>[2x]MSKQGLTAGLAEAVRTSQPEHSVDAIRKAKKGLLDFTAASFAGR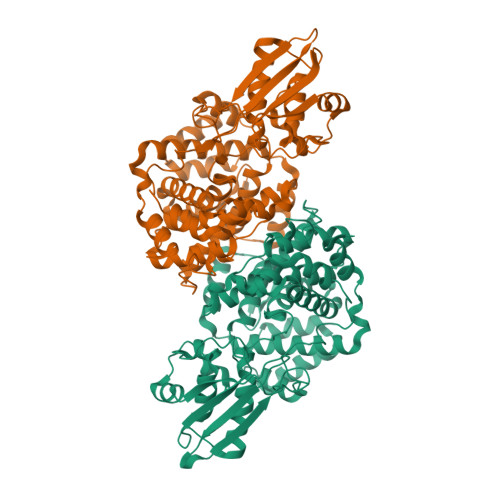EDKGIQKLLRLIEDEGGRPLVPIIGQGKKAAPLQSAMLNGFIAHALDFDDVHSDVRGAPSAVIVPALIASAARGHDERLLGAYIVGVEVMARLGESIGSRHYEKGWHNTGTLGAIAAACAVGYAEELTQEELEKAIGFAATQSAGMRVQFGTEMKPLHAGLAAQAGLLAVKLAQSEFGGSRTAFDGETGFFSLYGDVEKAQHTLLNDWGAPWRIVQPGLWFKIYPFCSAAHHAADAVRQLISEETISAANTERIEVIFPPGGDAALTERSPKTGEEGRFSVEYVIALALHGHGLTVEHFSSQPIPNGIQTTIGHIQRVYDNATQPAPHAVPKGRFTIVRAYLSDGRICEARVDCPKGAPGNELSEEDIIEKLTLTVPQEKARRIITAVEKADIKEFLAHIELEHHHHHH>TGTQRFKEALQDPFTLCLANVPGQPDLRHIVIDGSNVAMVHGLQHYFSSRGIAIAVQYFWDRGHRDITVFVPQWRFSKDAKVRESHFLQKLYSLSLLSLTPSRVMDGKRISSYDDRFMVKLAEETDGIIVSNDQFRDLAEESEKWMAIIRERLLPFTFVGNLFMV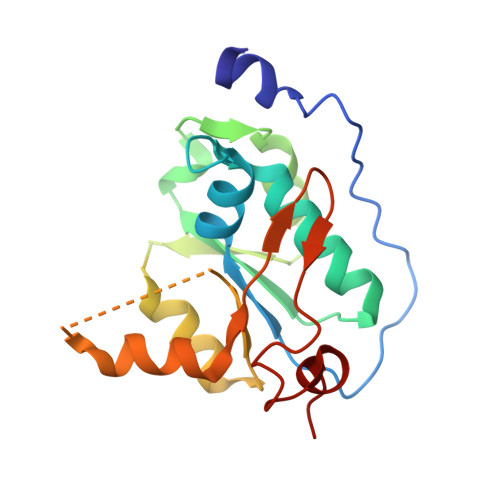PDDPLGRNGPTLDEFLKKP[2x]> SGGGMLTLIQGKKIVNHLRSRLAFEYNGQLIKILSKNIVAVGSLRREEKMLNDVDLLIIVPEKKLLKHVLPNIRIKGLSFSVKVCGERKCVLFIEWEKKTYQLDLFTALA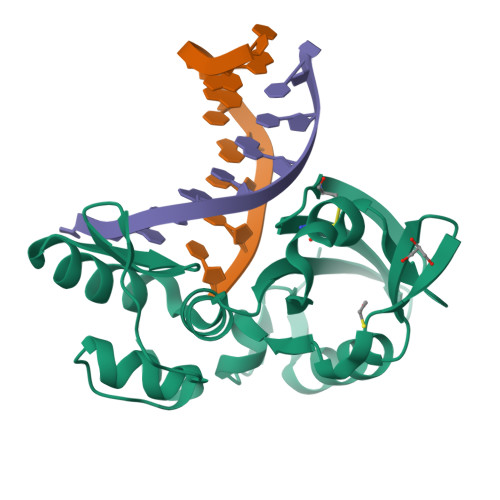EEKPYAIFHFTGPVSYLIRIRAALKKKNYKLNQYGLFKNQTLVPLKITTEKELIKELGFTYRIPKKRL6-[1-(2,2-difluoroethyl)-4-(6-methylpyridin-2-yl)-1H-imidazol-5-yl]imidazo[1,2-a]pyridine 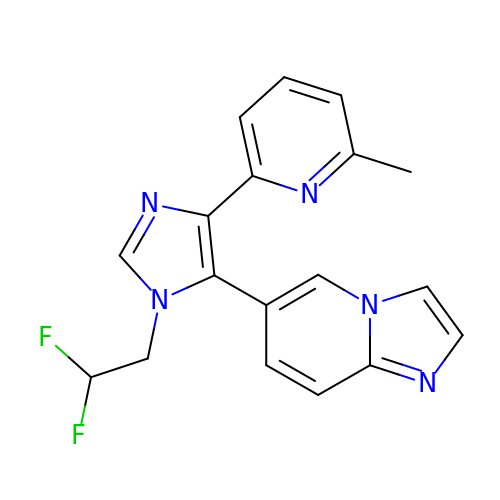| C18 H15 F2 N5 | WLMJUROXDOGLTR-UHFFFAOYSA-N>MAPVKVFGPAMSTNVARVTLCLEEVGAEYEVVNIDFNTMEHKSPEHLARNPFGQIPAFQDGDLLLWESRAISKYVLRKYKTDEVDLLRESNLEEAAMVDVWTEVDAHTYNPALSPIVYQCLFNPMMRGLPTDEKVVAESLEKLKKVLEVYE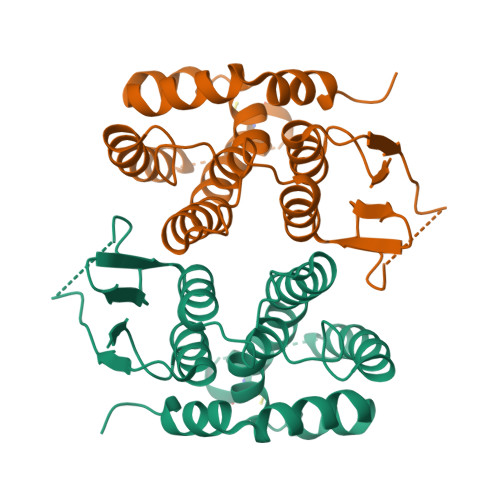ARLSKHSYLAGDFVSFADLNHFPYTFYFMATPHAALFDSYPHVKAWWDRLMARPAVKKIAATMVPPKA[6x]> MAIASEFSSLPSYAAFATAQEAYEQAVANGDSEVVLKKLKKSLNVAKSEFDRDAAMQRKLEKMADQAMTQMYKQARSEDKRAKVTSAMQTMLFTMLRKLDNDALNNIINNARDGCVPLNIIPLTTAAKLMVVIPDYNTYKNTCDGTTFTYASALWEIQQVVDADSKIV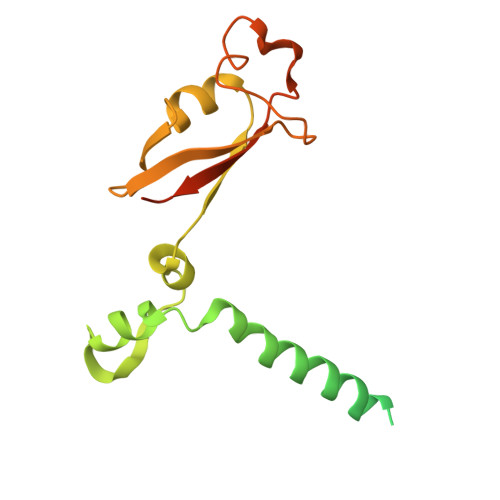QLSEISMDNSPNLAWPLIVTALRANSAVKLQLEHHHHHH> GSILDGPYQPTTFKPPNDYWLLISSNTDGVVYESTNNSDFWTAVIAVEPHVSQTNRQYVLFGENKQFNVENSSDKWKFFEMFKGSSQSDFSNRRTLTSNNRLVGMLKYGGRVWTFHGETPRATTDSSNTADLNNISIIIHSEFYIIPRSQESKCNEYINNGL

RV is a non-enveloped double-stranded RNA (dsRNA) virus with three concentric capsid layers encapsidating eleven dsRNA segments. The outermost layer contains the glycoprotein VP7 and the protease-sensitive spike protein VP4, which define the classification of RVs into G and P genotypes, respectively. RVs use the VP8* domain of the spike protein VP4 to recognize specific host glycans in a genotype-dependent manner. Our studies show that VP8* of these genotypes engages the type I precursor glycan (Galβ1,3-GlcNAc) at a unique and conserved binding site that is present in all P, P and P HRVs, and the subtle sequence and structural changes lead to an altered glycan configuration at the reducing end in the neonate-specific P RV, that may play a key role in the age-restricted tropism of some P strains.

However, although the VP8* structures of P HRV (DS-1-like) and P HRV (Wa-like) in isolation have been determined, it is not known how they bind to cellular glycans due to the lack of their structures in complex with any glycans. To investigate how other prevalent HRV strains recognize type I glycans, we determined the crystal structure of VP8* of a G2P HRV alone and in complex with H-type I pentasaccharide at 1.6 and 1.3 Å, respectively.> MRIGITYTVLRREEMAIKERAGEFGEVV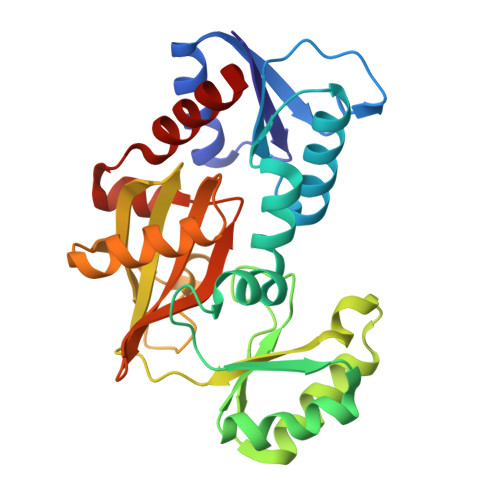MLHEDDLLFPGNYDLDVVIIRNVSHFKALYTARLFESEGIPTVNSSRLIFEAGDKLFATLRLAGKVPVPEWKAALSEGGALRVPDSLGYPLVSKPVFGSWGRLLAKVNDRDSLEAVLEHRKWMKNPLYGIHYFQEFVEKPGRDIRSYVIGGEFVGAIYRYSNHWITNTARGGKAEPCSDPEVEELSVKAWEAFGEGALAIDIFESEKGLLVNEVNPNMEFKNAARVTGADMAGKLVEYAVEVAKT> MPGFNYGGKGDGTGWSSERGSGPEPGGGSHGNSGGHDRGDSSNVGNESVTVMKP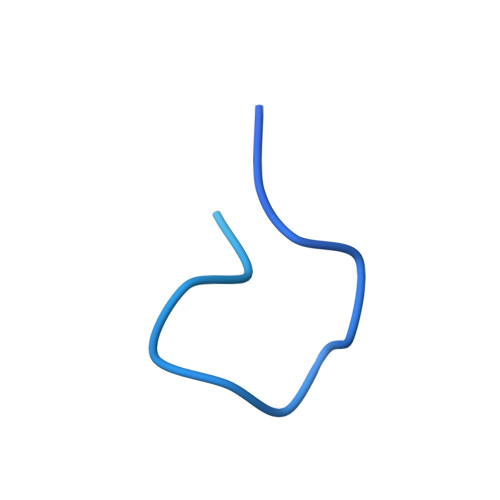GDSYNTPWGKVIINAAGQPTMNGTVMTADNSSMVPYGRGFTRVLNSLVNNPVSLEHHHHHH> PDYVFHRAHERMLFQTSYTLENNGSVICIPNNGQCFCLAWLKSNGTNAEKLAANILQWITFALSALCLMFYGYQTWKSTCGWEEIYVATIEMIKFIIEYFHEFDEPAVIYSSNGNKTVWLRYAEWLLTCPVILIHLSNLTGLANDYNKRTMGLLVS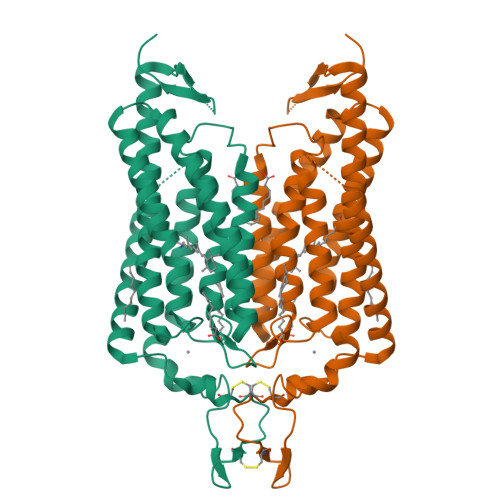DIGGIVWATTAALSKGYVRVIFFLMGLCYGIYTFFNAAKVYIEAYHTVPKGRCRQVVTGMAWLFFVSWGMFPILFILGPEGFGVLSVYGSTVGHTIIDLMSKNCWGLLGHYLRVLIHEHILIHGDIRKTTKLNIGGTEIEVETLVEDE> ADD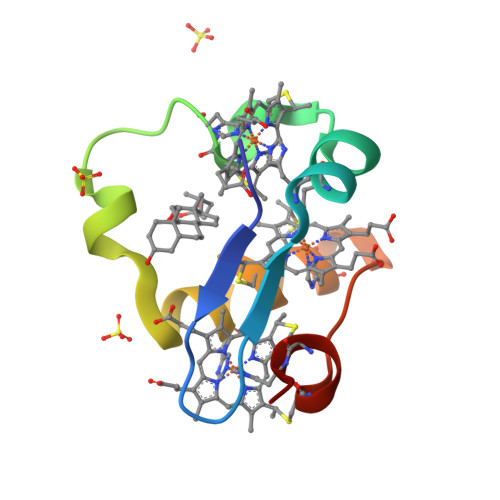IVLKAKNGDVKFPHKAHQEAVPDCKKCHEKGPGKIEGFGKEMAHGKGCKGCHEEMKKGPTKCGECHKK> MQAIKESYAFAVLGEPRYAFNFNHFDYVNPAAPKGGQITLSALGTFDNFNRYALRGNPGARTEQLYDTLFTTSDDEPGSYYPLIAESARYADDYSWVEVAINPRARFHDGSPITARDVEFTFQKFMTEGVPQFRLVYKGTTVKAIAPLTVRIELAKPGKEDMLSLFSLPVFPEKYWKDHKLSDPLATPPLASGPYRVTSWKMGQNIVYSR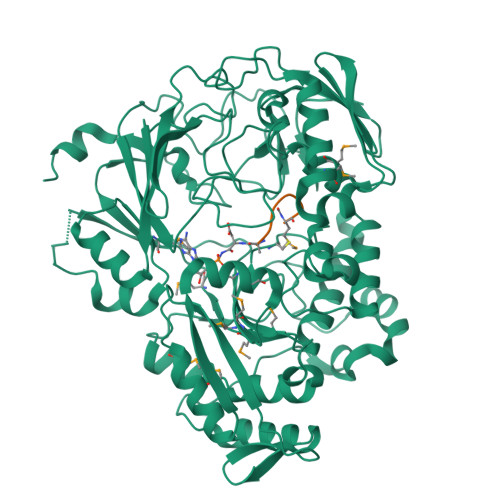VKDYWAANLPVNRGRWNFDTIRYDYYLDDNVAFEAFKAGAFDLRMENDAKNWATRYTGKNFDKKYIIKDEQKNESAQDTRWLAFNIQRPVFSDRRVREAITLAFDFEWMNKALFYNAWSRTNSYFQNTEYAARNYPDAAELVLLAPMKKDLPSEVFTQIYQPPVSKGDGYDRDNLLKADKLLNEAGWVLKGQQRVNATTGQPLSFELLLPASSNSQWVLPFQHSLQRLGINMDIRKVDNSQITNRMRSRDYDMMPRVWRAMPWPSSDLQIAWSSEYINSTYNAPGVQSPVIDSLINQIIAAQGNKEKLLPLGRALDRVLTWNYYMLPMWYMAEDRLAWWDKFSQPAVRPIYSLGIDTWWYDVNKAAKLPSASKQGE;> MRTGNAX> DTELNIENEAKLFKNLTFYLYEFPNTKVSRLHKCLSDN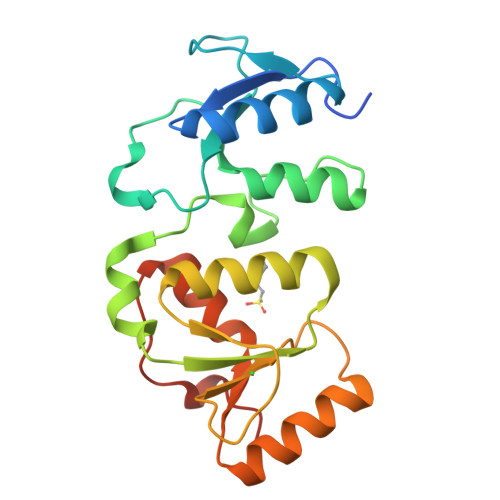GGQISEFLSSTIDFVVIPHYFPVDELPIFSFPTVNEWWIERCLYYKKIFGIDEHALAKPFFRPSLVPYFNGLSIHLTGFKGEELSHLKKALTILGAVVHEFLGVQRSILLVNTNEPFSMKTRFKIQHATEWNVRVVGVAWLWNIIQSGKFIDQVSPWAIDKKENQE> MKTLGEFIVEKQHEFSHATGELTALLSAIKLGAKIIHRDINKAG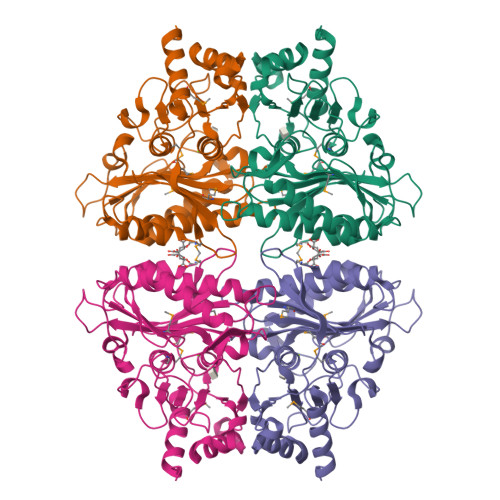LVDILGASGAENVQGEVQQKLDLFANEKLKAALKARDIVAGIASEEEDEIVVFEGCEHAKYVVLMDPLDGSSNIDVNVSVGTIFSIYRRVTPVGTPVTEEDFLQPGNKQVAAGYVVYGSSTMLVYTTGCGVHAFTYDPSLGVFCLCQERMRFPEKGKTYSINEGNYIKFPNGVKKYIKFCQEEDKSTNRPYTSRYIGSLVADFHRNLLKGGIYLYPSTASHPDGKLRLLYECNPMAFLAEQAGGKASDGKERILDIIPETLHQRRSFFVGNDHMVEDVERFIREFPDA> LNTIDIQGDILVGMHKQKQLFYFFAINDPATFKTHLASDIAPVVASVTQLSNVATQPLVALNIAFSNTGLLALGVTDNLGDSLFANGQAKDATSFKESTSSWVPQFAGTGIHGVIILASDTTDLIDQQVASIESTFGSSISKLYSLSASIRPGNEAGHEMFGFLDGIAQPAINGFNTPLPGQNIVDAGVIITGATNDPITRPSWAVGGSFLAFRQLEQLVPEFNKYLLDNAPAGSGSLQARADLLGARMVGRWKSGAPIDLTPTADDPALGADAQRNNNFTYSHAGFDLGSDQSH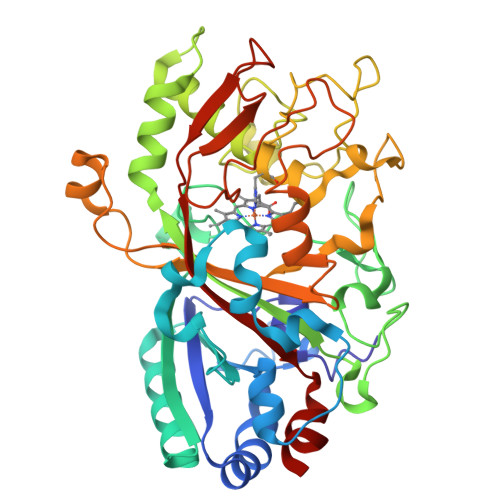CPFSAHIRKTRPRADLGGSLTPPNLSAGANSIMRSGIPYGPEVTSAESASNTTTQERGGAFVAYQAQLSQGFHFLQQTWADNANFPPGKTPATVGLDPIIGQNNGQPRVVNGLLPSNSSASLSIPQFVVSHGGEYFFSPPISAIGGRLSA> MAHHHHHHMLIQRGGLKVVAGLGISGVSAVNFLHEQGYQVAVTDSRPTPPGHDQIPAGVKTSFGQLDQELLLQAEEIILSPGLAPQLPEIQAAIAKGISVVGDIQLLRRATDVPIVAITGSNAKSTVTTLIGLMAKDAGKKVAVGGNLGRPALDLLKDQPELLVLELSSFQLETTSHLNAEVAVVLNMSEDHLDRHGNMLGYHQAKHRIFQGAKKVVFNRDDALSRPLVPDTTPMQSFGLNAPDLNQYGVLRDADGTLWLARGLQRLIKSSDLYIQGMHNVANALACLALGEA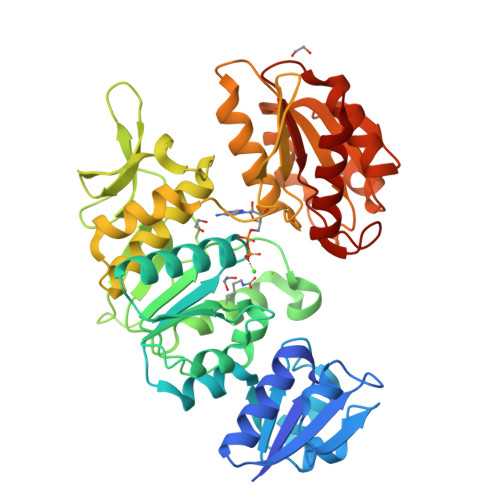IGLPMESMLETLKQFKGLEHRCEYVKTVHDVRYYNDSKGTNVGATLAAIDGLGAAIEVKKGKVALILGGQGKGQDFGPLRSSIEKYAKVVVLIGEDAPVIEQAIQGATKILHAATLKEAVELCQRETQAEDVVLLSPACASFDMFKSYNDRGQQFVACVNSLV Guaijaverin | C20 H18 O11 | 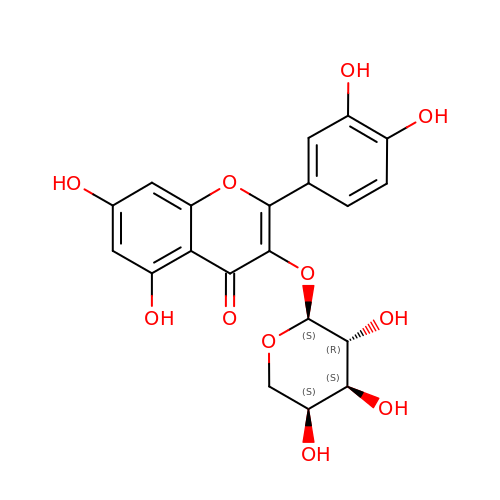PZZRDJXEMZMZFD-IEGSVRCHSA-N>[2x]GPEFRNEIRQKINPYRSHMKQKFQVLWEKEPCLLVPEDFYEETTKIEYELLSTVYLDAFKPGESSPTVVLHGPEGIGKTTFLRKVML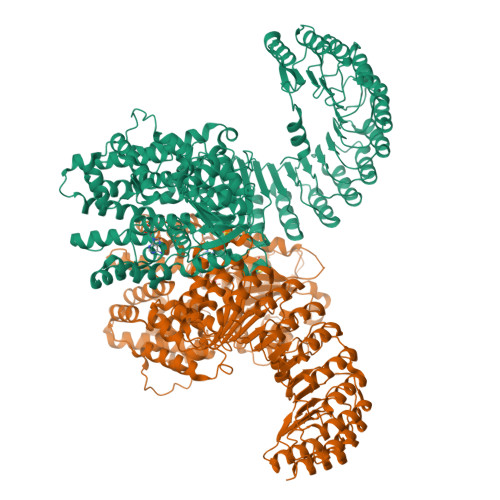EWAKGNLWRDRFSFVFFLTGREMNGVTDMSLVELLSRDWPESSEPIEDIFSQPERILFILDGMEELKFDLDCNADLCEDWEQPQSMQVVLQSLLQKQMLPECSLLLALSKMGMRKNYSLLKHMKCIFLLGFSEHQRKLYFSHYFQEKDASSRAFSFVREKSSLFVLCQSPFLCWLVCTSLKCQLEKGEDLELDSETITGLYVSFFTKVFRSGSETCPLKQRRARLKSLCTLAAEGMWTCTFLFCPEDLRRNGVSESDTSMWLDMKLLHRSGDCLAFIHTCIQEFCAAMFYMFTRPKDPPHSVIGNVTQLITRAVSGHYSRLSWTAVFLFVFSTERMTHRLETSFGFPLSKEIKQEITQSLDTLSQCDPNNVMMSFQALFNCLFETQDPEFVAQVVNFFKDIDIYIGTKEELIICAACLRHCHSLQKFHLCMEHVFPDESGCISNTIEKLTLWRDVCSAFAASEDFEILNLDNCRFDEPSLAVLCRTLSQPVCKLRKFVCNFASNLANSLELFKVILHNPHLKHLNFYGSSLSHMDARQLCEALKHPMCNIEELMLGKCDITGEACEDIASVLVHNKKLNLLSLCENALKDDGVLVLCEALKNPDCALEALLLSHCCFSSAACDHLSQVLLYNRSLTFLDLGSNVLKDEGVTTLCESLKHPSCNLQELWLMNCYFTSVCCVDIATVLIHSEKLKTLKLGNNKIYDAGAKQLCKALKHPKCKLENLGLEACELSPASCEDLASALTTCKSLTCVNLEWITLDYDGAAVLCEALVSLECSLQLLGLNKSSYDEEIKMMLTQVEEMNPNLIISHHLWTDDEGRRRGILV>[6x]MKLIDKLPSFDRNYIVEEIQGAYDTELNILKEDIDDTFNQLFVDTATWGLDMWEDILCIEKKELDFDTRRSNIKAKMRSRGTSTIEVIKSICEAYTKSETDIKVYSDEFTFVLSFIANNCDYKTLLDCSDMIERVKPAHLLHYLEPIILDKSMVYCGGGMVCSEEVKVHPYFEPIIKCSAVVNCGAGMISREEIKVYPLSIKCIENNCKINIAIANDTGVENVVVYPKSEVV;>MYSDQTYEVIKNRTLENINLDIYKGEGSFLNNMVSGNNLELSKIYLELSKMHKMAFIQDTYNQFLDKRVNEFGVYRKLGTESNGEVEFIGEKGTVINNGTIISYRDLLFVVIKDVTIGSEEGDNSPVQALEVGKKYNLPTNCEFKLVDNISGVTKITNTRSFEGGTDIETDEELKERFYKIQRNQATSGNKAHYEEWALEVDGVYNVKVYPRWDGPGTVKVLIFGKNNQAVDTETIERCQQHIDEEKPIGPTITVVTPLPIEISISAVMKLEDGYTLDNVKESFLESINTYFRDIRGEIIYTKVMGILINTTGVHDLSNLLINGSTDNITINEDKIPSVTTVNFSEVENQ[12x];>MAIGLPSINISFKELATTVKERSARGIIAMVLKDAKALGLNEIHEKEDIPVDLSAENKEYINLALMGNVNTPNKLLVYVIEGEADIQTALDFLETKEFNYLCMPKAVEADKTAIKNWIIKLRDIDKVKVKAVLGKVVGNHEGIINFTTEDVLVGEKKYSVDEFTSRVAGLIAGTPLSQSVTYTKLSDVVDIPKMTKVDAESRVNKGELILIKEAGAIRIARGVNSLTELTAEKGEMFQKIKIVDTLDIIHSDIRKVIIDDYIGKVTNSYDNKCLLIVAIKSYLEELEKSALIESDSTVEIDFEAQKSYLKSKGVDLSYMTLQEIKEANTGSKVFLKAKIKVLDAMEDIDLSIEI[18x];>[6x]MSTIFPFIGVPEDYILPKTEELPIFREVAWDFEKDEPILEKGDFKIIEKKEALKVWIYKCIKTNRYEHEIYSLEYGTELSELIGQKYTKGLTESEASRFIKEALLINPYILEVNVKSANFNRDILSANVKVSTIYGEVEINV

Here, we report the atomic structures of an engineered diffocin, a contractile syringe-like molecular machine that kills the Gram-positive bacterium Clostridioides difficile. Captured in one pre-contraction and two post-contraction states, each structure fashions six proteins in the bacteria-targeting baseplate, two proteins in the energy-storing trunk, and a collar linking the sheath with the membrane-penetrating tube. Specific attachment of baseplate tail fibers to receptors on the surface of a target bacterial cell triggers conformational changes of the neighboring baseplate, which leads to reorientation of sheath proteins and contraction of the entire sheath assembly. Since the sheath and the tube are anchored together at the opposite end by the collar, collapsing the sheath pushes the tube through the baseplate, driving it to puncture the cell wall and underlying cytoplasmic membrane.

CryoEM data processing of the post-contraction diffocin particles resolved two different substates, an apparent transitional state and a final state, which is 2 nm shorter in length. Using the same strategy, we determined the cryoEM structures of the collar, trunk, and baseplate in the transitional and final states at 3.6–6.1 Å resolution. The baseplate wedges in the transitional and final states are almost identical, with both presenting a post-contraction conformation. By comparing them to the pre-contraction baseplate wedge, we observed repositioning of the dimerization domains of Tri2A and Tri2B, along with a twist of the trifurcation unit relative to the core bundle; the dimer interface between neighboring triplexes is, however, preserved. These movements result in an expansion of the iris ring from 24 to 26 nm, with the ring structure remaining intact. Although the conformational change in the diffocin baseplate wedge is less dramatic than in R-type pyocin, where the iris ring breaks apart after contraction, it is still sufficient to initiate the contraction and release the bound hydrolase domain of the hub-hydrolase. The observation that sheath layers on the baseplate side are fully contracted, while those on the collar side are partially contracted, supports the wave-like propagation model from the baseplate to the collar, and our structure of the diffocin in the transitional state provides atomic resolution details of a intermediate of potential relevance to other Gram-positive CISs. After contraction to the transitional state, the tube protrudes 45 nm away from the baseplate. We did not observe the density of the hydrolase domains at the spike-proximal tube region in the post-contraction state due to the limited number of particles.IAV contains two glycoproteins with different functional roles; HA binds to sialoglycan receptors and mediates membrane fusion, whereas neuraminidase (NA) is the receptor-destroying enzyme that removes the terminal sialic acids. The sialidase activity of NA is essential for virion release from (decoy) receptors on host cells and for virion mobility through sialic acid-dense surroundings to reach functional entry receptors. The tetrameric NA protein consists of a globular head domain, containing the catalytic site, a narrow stalk, a transmembrane region, and a short cytoplasmic domain. However, antibodies against neuraminidase (NA) can also confer protection against influenza, making NA an attractive target for the development of novel vaccines.

We produced soluble recombinant tetrameric NA proteins stabilized with a tetrabrachion tetramerization domain, validated their quaternary structure by cryo-electron microscopy (cryo-EM) single-particle analysis, and conjugated these to Mi3 self-assembling protein nanoparticles using the SpyTag-SpyCatcher system. The structural integrity of recombinant NA antigens is of critical importance for inducing an optimal immune response. It was recently shown that recombinant soluble tetrameric NAs, particularly of the N1 subtype, may suffer from structural instability in the head domain, resulting in an “open” conformation not generally observed on virions. Therefore, we performed cryo-EM to evaluate the quaternary structure of our constructs. 2D classification of the tetrabrachion-stabilized recombinant N1 NC13 produced class averages corresponding to different views of the NA tetramers, all of which were consistent with the closed conformation. The 3D reconstruction further confirmed this view. Collectively, these observations indicate that our NA antigens adopt a closed conformation similar to the presumed conformation of NA on viral particles. In contrast, our NA antigens adopt the closed conformation without the need for stabilizing mutations. This difference may be attributed to the different tetramerization domains that were used. The antigens were produced in a mammalian (HEK293F) expression system, affinity purified, and evaluated for purity and size on SDS-PAGE. The recombinant N1 and N2 proteins were highly enzymatically active in an assay based on the cleavage of the small molecule substrate MUNANA.

>VKLAGNSSLCPVSGWAIYSKDNSVRIGSKGDVFVIREPFISCSPLECRTFFLTQGALLNDKHSNGTIKDRSPYRTLMSCPIGEVPSPYNSRFESVAWSASACHDGINWLTIGISGPDSGAVAVLKYNGIITDTIKSWRNNILRTQESECACVNGSCFTIMTDGPSDGQASYKIFRIEKGKIVKSVEMNAPNYHYEECSCYPDSSEITCVCRDNWHGSNRPWVSFNQNLEYQIGYICSGVFGDNPRPNDKTGSCGPVSSNGANGVKGFSFKYGNGVWIGRTKSISSRKGFEMIWDPNGWTGTDNNFSIKQDIVGINEWSGYSGSFVQHPELTGLDCIRPCFWVELIRGRPEENTIWTSGSSISFCGVNSDTVGWSWPDGAELPFTI[4x]(4S)-4-[(1R)-1-hydroxy-2-({[3-(propan-2-yl)phenyl]methyl}amino)ethyl]-19-(2-oxopropoxy)-11,16-dioxa-3-azatricyclo[15.3.1.1~6,10~]docosa-1(21),6(22),7,9,17,19-hexaen-2-one 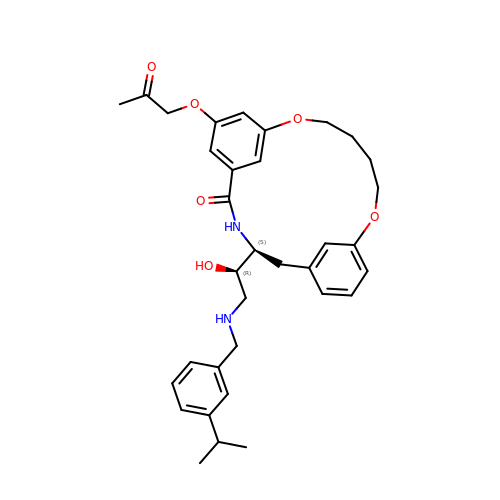| C34 H42 N2 O6 | MKUSLLRHQBCOIB-JHOUSYSJSA-N piperidine-1-carboximidamide | C6 H13 N3 | 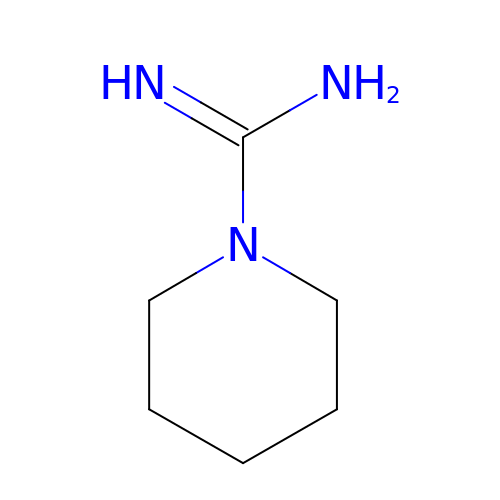QUUYRYYUKNNNNS-UHFFFAOYSA-N> NKTGITYPEIKLGETGKDIKTTITFMNNRTDMNLDTYPGKNWKSYIEDFNKMYPNITVKVQTDSNYADSALTRLQANNDSWDIMMIPAVDKSEFSNYFVPYGETSEMEKVIKLADEKAYDGQTYG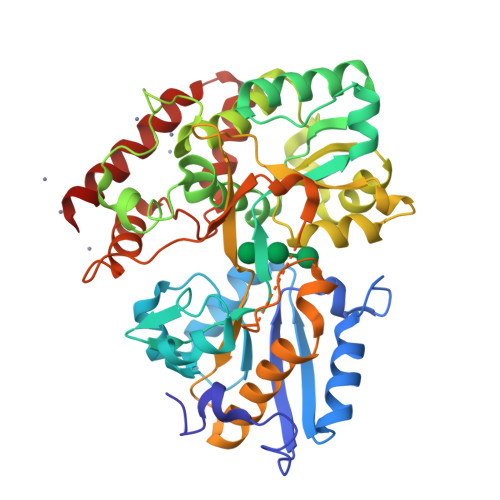IANNGVTAGIVYNKKVFEEAGIKELPKTPEEFQADLKLIKEKTKAVPLYTNFVEDWAMGAWDQYIAGNATGDPKFMNQVLPTTKEPFKKDASAPDTHPYAVYKTLYDAVANGYTEEDYSTTDWESSKGKMNNGEIATMVLGAWAVPQMKQAGDHPDDIGYMPFPITVDGKQYATIAGDYSYGINKNISKEKQEASMIFVKWMTEDSGFAKNEGGIPIKADDESMPETYETFSDVELITDAPAKEGQEDLLANVNSDSELGINNGNGKKIQDIVVDAANRTRTIDQIMDEWNQKWAKAVEDN>[2x]MGMKLLVVSWGDFERWKETKYRFGGETSVGPSTLPILQKVIKPDWTVIVLSDTIGKDFSSVETLREDVRNRVMDFLDRIGAGREVDVIIAPGIGEFTHGSFRGSAMDAYYYVLHALSEIIPTKGDLEVHFDSTAGLNYVTLLTYRALKD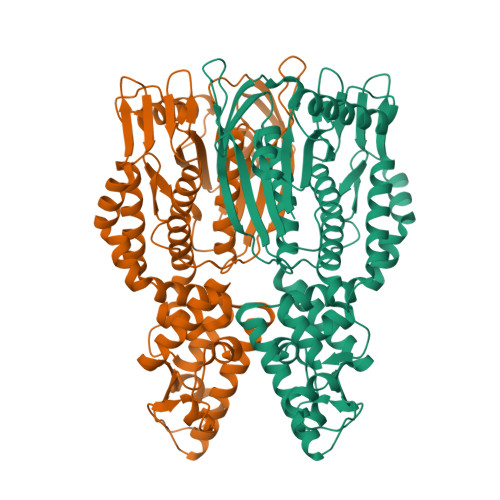LLGIAAVMNTVTFYAYNSDPFVPKITKELNINTIETTMVKPTPLSEPLPGFDEYLCPYSMERAEFVRLKGSLNTLKNLRKEKKKLEAWIGSLLFGLPLLFLEEFPDIGRLESYIEELAETWGGAIAVNAEEKAVTRRLAFGSGFGTLVKLLFQARITRGLLVEEPYSIEKLYSVSDRLFRGSTLQRVRVELGKIEDKAIKYARKGAFPRDIPLRDFLGFDAANREVSPRNVLAHAGLEANVVEVSMEAWEPKRPEEEAGRHTHLKYTPVGLKKVEDIVSRALKESHHHHHH> SLMKKRRNWHRHDYTEIDDGSKPVQAGTRTFIKELRSRVFPSADEIIIKMHGSQ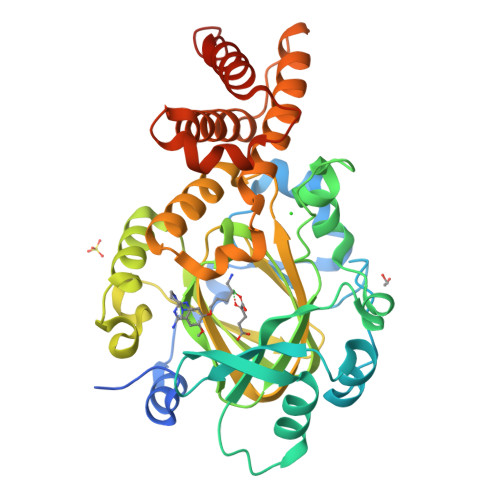LTQRYLEKHGFDVPIMVPKLDDLGLRLPSPTFSVMDVERYVGGDKVIDVIDVARQADSKMTLHNYVKYFMNPNRPKVLNVISLEFSDTKMSELVEVPDIAKKLSWVENYWPDDSVFPKPFVQKYCLMGVQDSYTDFHIDFGGTSVWYHVLWGEKIFYLIKPTDENLARYESWSSSVTQSEVFFGDKVDKCYKCVVKQGHTLFVPTGWIHAVLTSQDCMAFGGNFLHNLNIGMQLRCYEMEKRLKTPDLFKFPFFEAICWFVAKNLLETLKELREDGFQPQTYLVQGVKALHTALKLWMKKELVSEHAFEIPDNVRPGHLIKELSKVIRAIEEENGKPVKSQGI>MHHHHHHSSGRENLYFQGAAPPSTREMVQLVDSLNRREDGGAFSVDVAEAYPDLRDSYRKICPRPMNLILMRQRAKEGYYTSGSATVYGDTVAASLTRLREDIELLVRNCITFNVKVESWVTLARSFQAFAH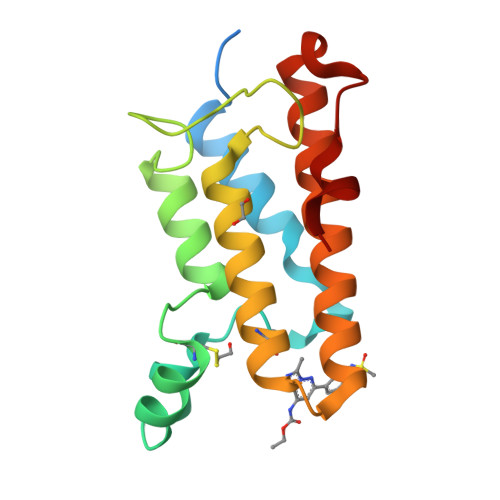RRVDDFVLRHAAFLRGTTMGAEVYE[2x]N-[3-(tert-butylamino)propyl]-3-(trifluoromethyl)benzamide 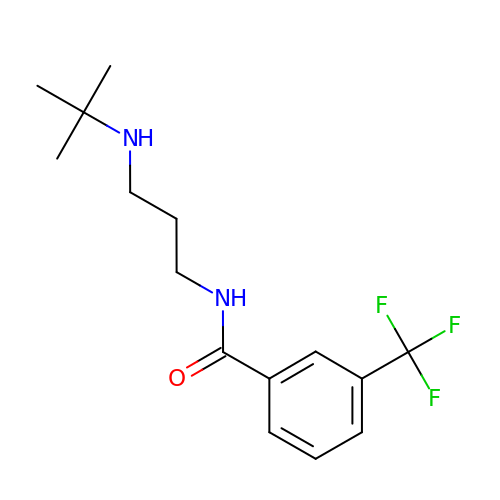| C15 H21 F3 N2 O | UTBTYWGTMLPLJP-UHFFFAOYSA-N> GPMEEIRNLTVKDFRVQELPLARIKKIMKLDEDVK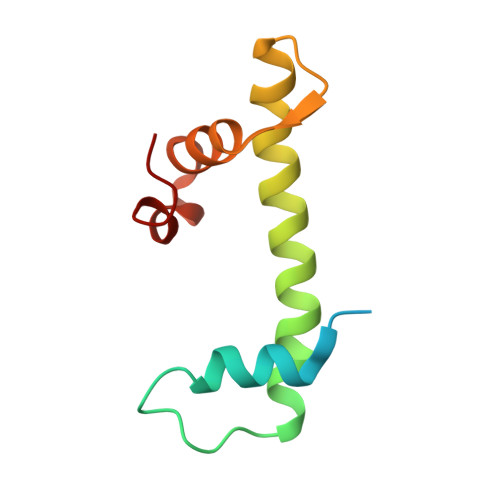MISAEAPVLFAKAAQIFITELTLRAWIHTEDNKRRTLQRNDIAMAITKFDQFDFLIDIVPR>[2x]GTEDTVIKVSVLRGPSVIAFADWLENPPIIDNKKVQVKVVDSPDLAQALLIKQETDIAVLPMINAANLYNKGIKIKLAGCPIWGTLYLVEKTPLKEPALYVFGNGTTPDILTRYYLGR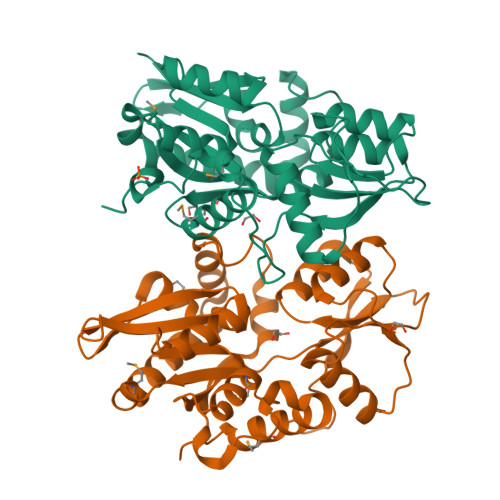QRLDYPLNYAFNTAGEITQGILAGKVNRAVLGEPFLSIALRKDSSLRITADLNHLTDNDTLGFAQTAVVYTPTMEKYRIAFEDALRASCQKAVRYPKETIHSLEEHGIFAQGALTPKSIERCKIYYLSAIEAKDAVMGFLRLIEQYEPKAVGGRLPDAGFIPEKQ>MKVLVTGFEPFGGEKINPTERIAKDLDGIKIGDAQVFGRVLPVVFGKAKEVLEKTLEEIKPDIAIHVGLAPGRSAISIERIAVNAIDARIPDNEGKKIEDEPIVPGAPTAYFSTLPIKKIMKKLHERGIPAYISNSAGLYLCNYVMYLSLHHSATKGYPKMSGFIHVPYIPEQIIDKI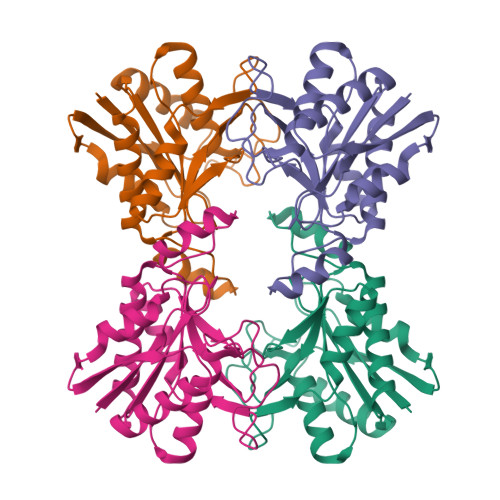GKGQVPPSMCYEMELEAVKVAIEVALEELL[4x]>MSDSHHKPVWDRTHHAKMATGIGDPQCFKGMAGKSKFNVGDRVRIKDLPDLFYTRTMTYTRGATGTIVRLVYESPAAEDEAFGNEENVEWFYSIVFAQKDLWPEYSDTFANDTLETEIPERYLEKA[4x];>[4x]MSSSIREEVHRHLGTVALMQPALHQQTHAPAPTEITHTLFRAYTRVPHDVGGEADVPIEYHEKEEEIWELNTFATCECLAWRGVWTAEERRRKQNCDVGQTVYLGMPYYGRWLLTAARILVDKQFVTLTELHNKIVEMRERVASGQGLGEYLPPKAK;>[4x]MSADHDHDHDHDHDHKPAPMVEEVSDFEILEMAVRELAIEKGLFSAEDHRVWKDYVHTLGPLPAARLVAKAWLDPEYKKLCIEDGVEASKAVGVNWVTSPPTQFGTPSDYCNLRVLADSPTLKHVVVCTLCSCYPRPILGQSPEWYRSPNYRRRLVRWPRQVLAEFGLQLPSEVQIRVADSNQKTRYIVMPVRPEGTDGWTEDQLAEIVTRDCLIGVAVPKPGITVNAKRPVLKANRPVHHD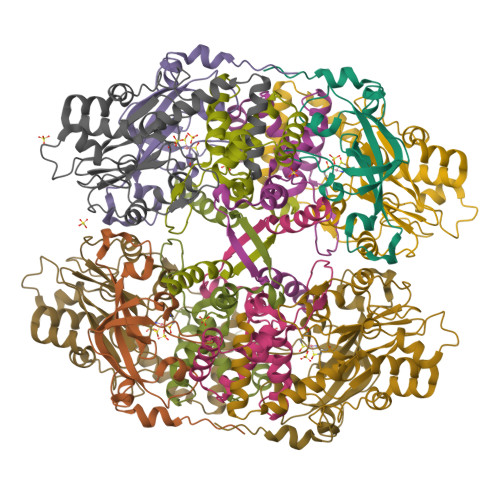H>[2x]MIILEKERVTVNPDIKVIKRDGRMVTFDSSKIYEAILKASETITPITPLIETKLEGIANRVVAEINDRFSHNIKIYEIQSIVEHELLEANEYAIAQEYINYRTKRDFERSQATDINFTINKLVNKDQAVVHENANKDSDLYNTQRDLTAGIVGKSVGLKMLPPHVANAHQKGDIHFHDLDYSPYTPMTNCCLIDFKGMLANGFKIGNAEVESPKSIQTATAQISQIIANVASSQYGGCTADRIDEFLAPYAELNYKKHLADAKEWVTEEKQEDYARAKTRKDIYDAMQSLEYEINTLFTSNGQ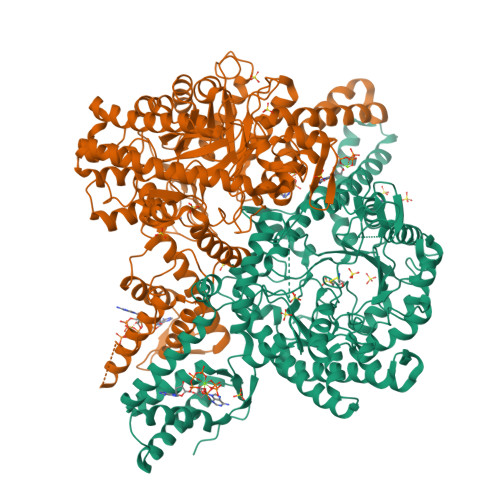TPFTSLGFGLGTNWFEREIQKAILQVRILGLGSEHRTAIFPKLIFTLKRGLNLEPNSPNYDIKQLALECATKRMYPDVLSYDKIIELTGSFKAPMGCRSFLQGWKDENGVEVNSGRMNLGVVTLNLPRIALESKGDQDKFWEIFEERMGIAKDALVYRVERVKEATPANAPILYQYGAFGQRLRKCDSVDQLFKHRRATVSLGYIGLYEVASVFYGSDWETNLEAKTFTLNIVKAMKNACESWSDEYDYHFSVYSTPSESLTDRFCRLDTEKFGVVTDITDKEYYTNSFHYDVRKNPTPFEKLEFEKDYPEAGATGGFIHYCEYPVLQQNPKALEAVWDFAYDRVGYLGTNTPIDKCYKCDFEGDFTPTERGFMCPNCGNTDPKTVDVVKRTCGYLGNPQARPMVKGRHKEISARVKHMNGSTIKYGGKHL>[4x]AQCSVDIQGNDQMQFNTNAITVDKSCKQFTVNLSQPGN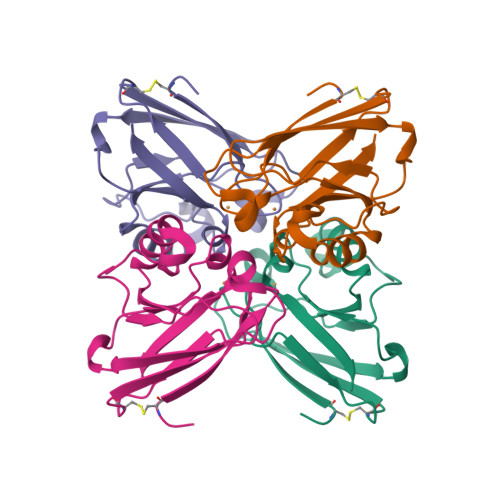LPKNVMGHNWVLSTAADMQGVVTDGMASGLDKDYLKPDDSRVIAHTKLIGSGEKDSVTFDVSKLKEGEQYMFFCTFPGHSALMKGTLTLK L-allose 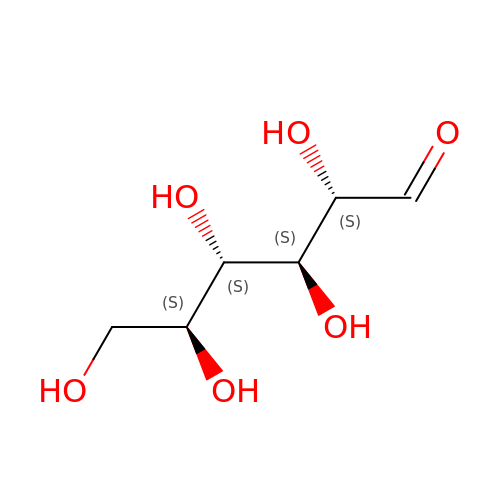| C6 H12 O6 | GZCGUPFRVQAUEE-MOJAZDJTSA-N>GVEEKKSLEILLKDDRLDTEKLCTFSQRFPLPSMYRALVWKVLLGILPPHHESHAKVMMYRKEQYLDVLHALKVVRFVSDATPQAEVYLRMYQLESGKLPRSPSFPLEPDDEV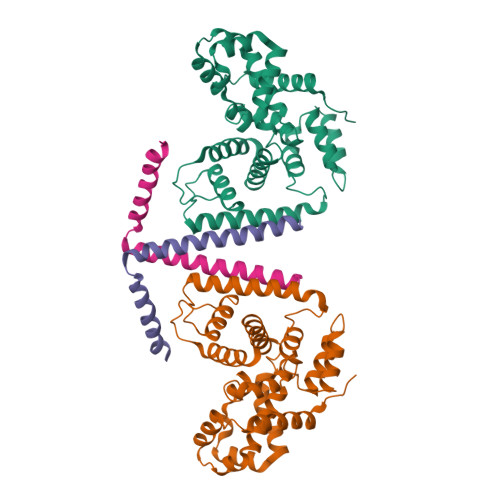FLAIAKAMEEMVEDSVDCYWITRRFVNQLNTKYRDSLPQLPKAFEQYLNLEDGRLLTHLRMCSAAPKLPYDLWFKRCFAGCLPESSLQRVWDKVVSGSCKILVFVAVEILLTFKIKVMALNSAEKITKFLENIPQDSSDAIVSKAIDLWHKHCGTPVHSS[4x];>[4x]RGQLQAAESRYEAQKRITQVFELEILDLYGRLEKDGLLKKLEEEKAEAAEAAEERL> GSMVEATAQETDRPRFSFSIAAREGKARTGTIEMKRGVIRTPAFMPVGTAATVKALKPETVRATGADIILGNTYHLMLRPGAERIAKLGGLHSFMGFDRPILTDSGGYQVMSLSSLTKQSEEGVTFK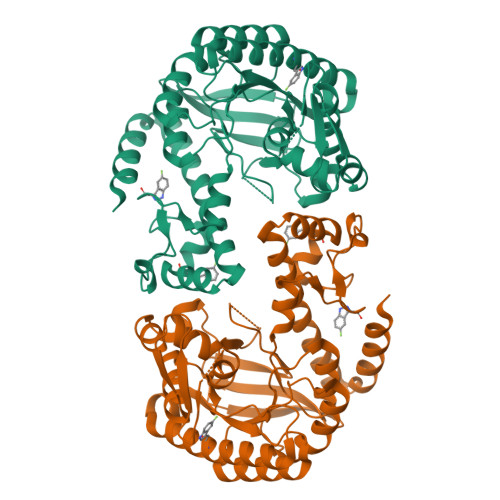SHLDGSRHMLSPERSIEIQHLLGSDIVMAFDECTPYPATPSRAASSMERSMRWAKRSRDAFDSRKEQAENAALFGIQQGSVFENLRQQSADALAEIGFDGYAVGGLAVGEGQDEMFRVLDFSVPMLPDDKPHYLMGVGKPDDIVGAVERGIDMFDCVLPTRSGRNGQAFTWDGPINIRNARFSEDLKPLDSECHCAVCQKWSRAYIHHLIRAGEILGAMLMTEHNIAFYQQLMQKIRDSISEGRFSQFAQDFRARYFARNS> MSEQEPYEWAKHLLDTKYIEKYNIQNSNTLPSPPGFEGNSSKGNVTRKQQDATSQTTSLAQKNQITVLQVQKAWQIALQPAKSIPMNIFMSYMSGTSLQIIPIMTALMLLSGPIKAIFSTRSAFKPVLGNKATQSQVQTAMFMYIVFQGVLMYIGYRKLNSMGLIPNAKGDWLPWERIAHYNNGL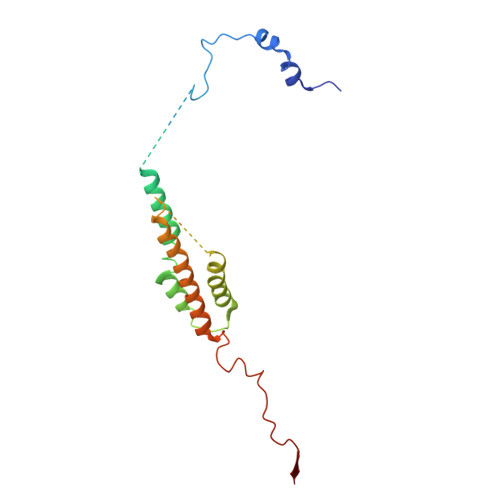QWFSD4,4'-bis(bromomethyl)biphenyl | C14 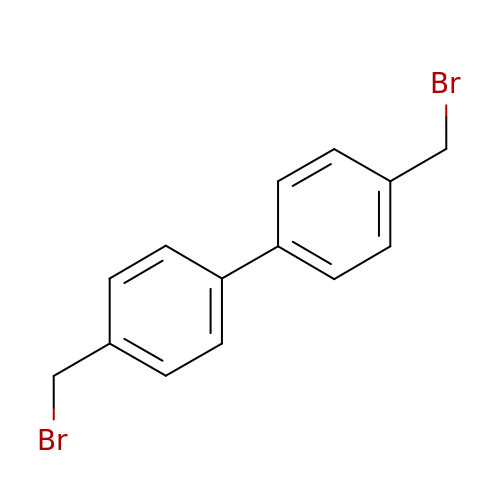H12 Br2 | HMUGRILXVBKBID-UHFFFAOYSA-N>[4x]MGSTSSLYAAIDLGSNSFHMLVVREVAGSIQTLTRIKRKVRLAAGLNSENALSNEAMERGWQCLRLFAERLQDIPPSQIRVVATATLRLAVNAGDFI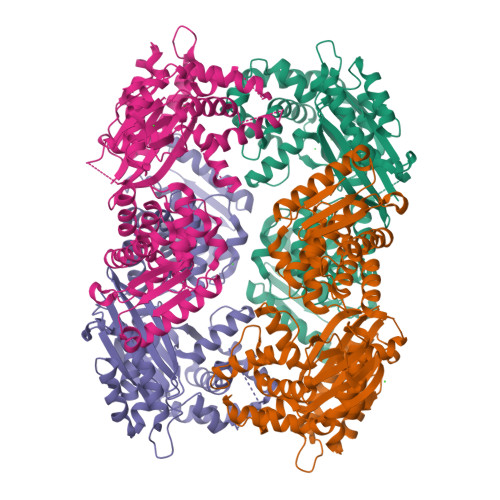AKAQEILGCPVQVISGEEEARLIYQGVAHTTGGADQRLVVDIGGASTELVTGTGAQTTSLFSLSMGCVTWLERYFADRNLGQENFDAAEKAAREVLRPVADELRYHGWKVCVGASGTVQALQEIMMAQGMDERITLEKLQQLKQRAIHCGRLEELEIDGLTLERALVFPSGLAILIAIFTELNIQCMTLAGGALREGLVYGMLHLAVEQDIRSRTLRNIQRRFMIDIDQAQRVAKVAANFFDQVENEWHLEAISRDLLISACQLHEIGLSVDFKQAPQHAAYLVRNLDLPGFTPAQKKLLATLLLNQTNPVDLSSLHQQNAVPPRVAEQLCRLLRLAIIFASRRRDDLVPEMTLQANHELLTLTLPQGWLTQHPLGKEIIAQESQWQSYVHWPLEVH>MEKDLLDKLGQHLVWRMGRAEDEDVLVVRVGLASATPRFRELPR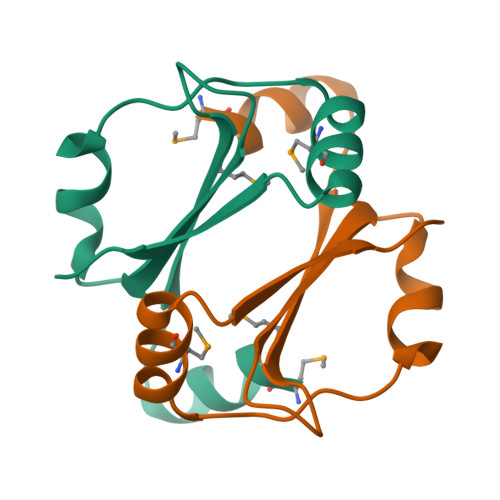LLNLPEAEMRRLVQEGRVRVEWVEE[4x]>[4x]MSVTIDHTTENAAPAQAAVSDRAWALFRALDGKGLVPDGYVEGWKKTFEEDFSPRRGAELVARAWTDPEFRQLLLTDGTAAVAQYGYLGPQGEYIVAVEDTPTLKNVIVCSLCSCTAWPILGLPPTWYKSFEYRARVVREPRKVLSEMG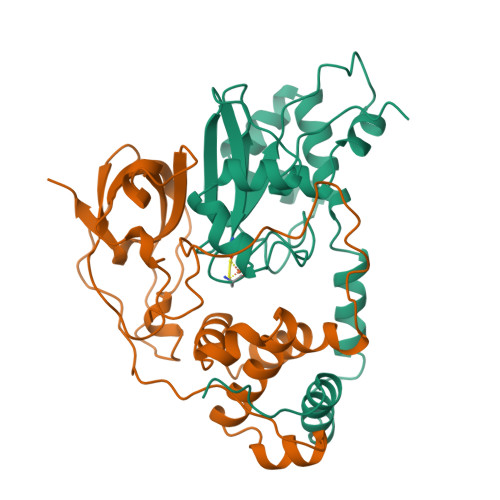TEIASDIEIRVYDTTAETRYMVLPQRPAGTEGWSQEQLQEIVTKDCLIGVAIPQVPTV;>[4x]MDGVHDLAGVQGFGKVPHTVDADIGPTFHAEWEHLPYSLMFAGVAELGAFSVDEVRYVVERMEPRHYMMTPYYERYVIGVATLMVEKGILTQDELESLAGGPFPLSRPSESEGRPAPVETTTFEVGQRVRVRDEYVPGHIRMPAYCRGRVGTISHRTTEKWPFPDAIGHGRNDAGEEPTYHVKFAAEELFGSDTDGGSVVVDLFEGYLEPAA>MFDLKKILDRPTIPWKLIISAFSIAQFSFESYLTYRQYQKLSETKLPPVLEDEIDDETFHKSRNYSRAKAKFSIFSDIYNLAQKLVFIKYDFFPKIWHMAVTLSNAVLPVRFHMVSTVAQSLCFLGLLSSMSTLVDLPLSYYSHFVLEEKFGFNKLTVKLWITDMIKSLTLAYAIGGPILYLFLKIFDKFPTDFLWYIMVFLFVVQILAMTIIPVFIMPLFNKFTPLEDGELKKSIESLADRVGFPLDKIFVIDGSKRSSHSNAYFTGLPFTSKRIVLFDTLVNSNSTDEITAVLAHEIGHWQKNHIVNMVIFSQLHTFLIFSLFTSIYRNSSFYNTFGFFVEKSSSGF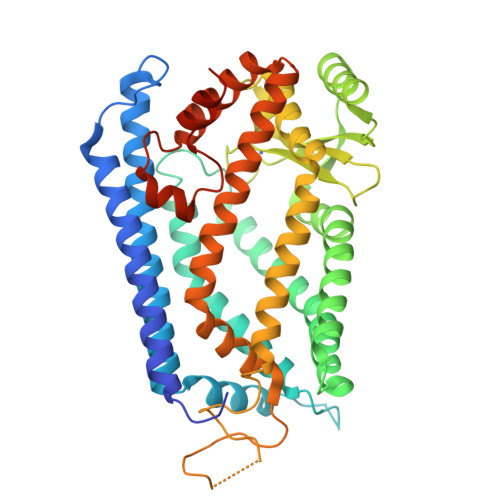VDPVITKEFPIIIGFMLFNDLLTPLECAMQFIMSLISRTHEYQADAYAKKLGYKQNLCRALIDLQIKNLSTMNVDPLYSSYHYSHPTLAERLTALDYVSEKKKNSGLEVLFQ[2x]Nevertheless, PBPs are still valid antibacterial drug targets as they are responsible for the vital crosslinking of peptidoglycan strands. The PBP3 structure contains a non-catalytic N-terminal domain and the C-terminal catalytic domain. Ideas for such different scaffolds often arose from β-lactamase inhibitor development efforts as serine β-lactamases and PBPs are evolutionarily related and share the same catalytic serine, other active site residues, and mechanism. To test whether the β-lactamase inhibitor vaborbactam can extend its inhibition ability to a homologous PBP, we probed the binding of vaborbactam to P. aeruginosa PBP3.

The cyclic boronic acid vaborbactam is bound in the active site in the same location as β-lactams such as ceftazidime and meropenem inhibiting this PBP3. Unbiased active site electron density shows vaborbactam covalently attached to the essential S294 in the catalytic domain; the boron bound to S294 is in sp3 configuration similar as observed when vaborbactam binds to serine β-lactamases. The hydroxyl moiety of the boronic acid is situated in the oxyanion hole. This hydroxyl moiety creates hydrogen bonding interactions with the backbone nitrogens of S294 and T487, with the hydroxyl of Y409, and with the backbone oxygen of T487. The amide oxygen of vaborbactam forms a hydrogen bond with the side chain nitrogen of N351; the amide nitrogen is hydrogen bonding with the backbone oxygen of T487. The carboxyl group of vaborbactam forms hydrogen bonds with T487, S485, and S349 and with water molecule W#1. The thiophene ring is seen forming hydrophobic interactions (< 4Å) with V333, Y503, and the T487 side chain. The carbon atoms of the boronate ring establish hydrophobic interactions with V333 and the Cβ atom of S349. Although both the aromatic wall (residues Y503, Y532, and F533) and hydrophobic bridge (V333 and F533) are formed upon vaborbactam binding, the crystallographically refined temperature factors of these residues are considerably higher compared to the core of the catalytic domain. Based upon these observations, we posit that the more mobile aromatic wall and hydrophobic bridge residues in the vaborbactam and zidebactam complexes are due to the presence of fewer hydrophobic moieties in these low affinity PBP3 inhibitors that could drive such stabilizing conformational changes (both inhibitors lack an R2 group).

> MGHHHHHHARSVRHIAIPAHRGLITDRNGEPLAVSTPVTTLWANPKELMTAKERWPQLAAALGQDTKLFADRIEQNAEREFIYLVRGLTPEQGEGVIALKVPGVYSIEEFRRFYPAGEVVAHAVGFTDVDDRGREGIELAFDEWLAGVPGKRQVLKDRRGRVIKDVQVTKNAKPGKTLALSIDLRLQYLAHRELRNALLENGAKAGSLVIMDVKTGEILAMTNQPTYNPNNRRNLQPAAMRNRAMIDVFEPGSTVKPFSMSAALASGRWKPSDIVDVYPGTLQIGRYTIRDVSRNSRQLDLTGILIKSSNVGISKIAFDIGAESIYSVMQQVGLGQDTGLGFPGERVGNLPNHRKWPKAETATLAYGYGLSVTAIQLAHAYAALANDGKSVPLSMTRVDRVPDGVQVISPEVASTVQGMLQQVVEAQGGVFRAQVPGYHAAGKSGTARKVSVGTKGYRENAYRSLFAGFAPATDPRIAMVVVIDEPSKAGYFGGLVSAPVFSKVMAGALRLMNVPPDNLPTATEQQQVNAAPAKGGRG> NAVVQLTELGNGVVQITMKDESSRNGFSPSIVEGLRHCFSVVAQNQQYKVVILTGYGNYFSSGASKEFLIRKTRGEVEVLDLSGLILDCEIPIIAAMQGHSFGGGLLLGLYADFVVFSQESVYATNFMKYGFTPVGATS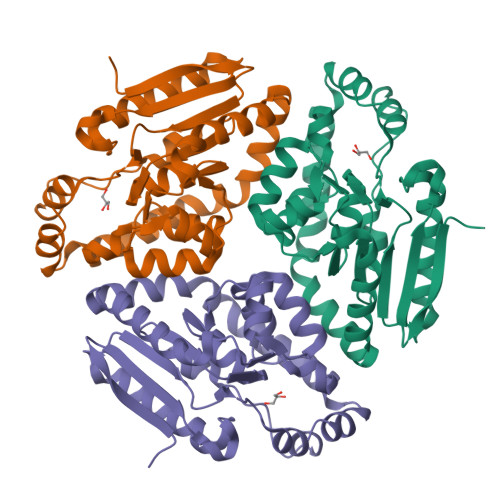LILREKLGSELAQEMIYTGENYRGKELAERGIPFPVVSRQDVLNYAQQLGQKIAKSPRLSLVALKQHLSADIKAKFPEAIKKELEIHQVTFNQPEIASRIQQEF2-[AMINO(IMINO)METHYL]-2-HYDROXYPHENOXY]-6-[3-(4,5-DIHYDRO-1H-IMIDAZOL-2-YL)PHENOXY]PYRIDINE-4-CARBOXYLIC 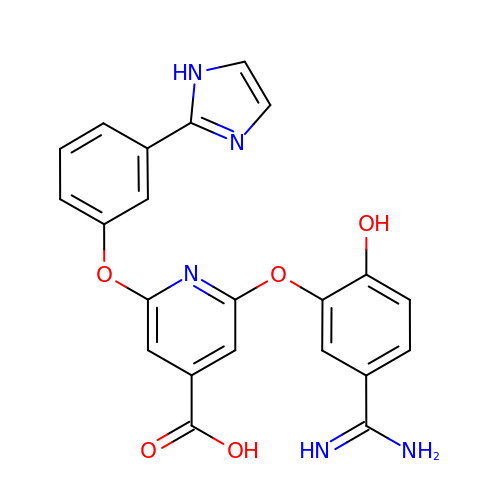ACID | C22 H17 N5 O5 | ILFWHJBPGCBXAY-UHFFFAOYSA-N> MKHGILVAYKPKGPTSHDVVDEVRKKLKTRKVGHGGTLDPFACGVLIIGVNQGTRILEFYKDLKKVFWVKMRLGLI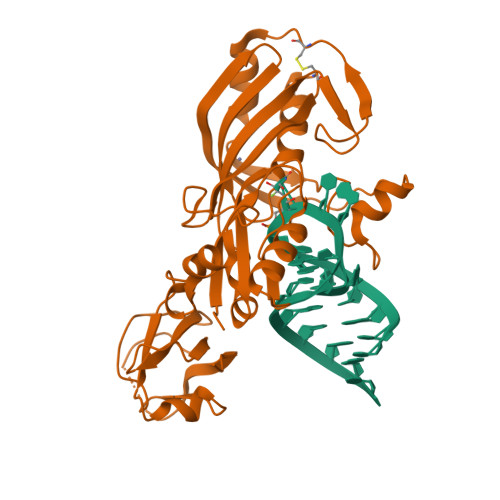TETFDITGEVVEERECNVTEEEIREAIFSFVGEYDQVPPAYSAKKYKGERLYKLAREGKIINLPPKRVKIFKIWDVNIEGRDVSFRVEVSPGTYIRSLCMDIGYKLGCGATAVELVRESVGPHTIEESLNVFEAAPEEIENRIIPLEKCLEWLPRVVVHQESTKMILNGSQIHLEMLKEWDGFKKGEVVRVFNEEGRLLALAEAERNSSFLETLRKHERQERVLTLRKVFQTR> MSEEKVVAVIMVGGPTKGTRFRPLSFNTPKPLIPLAGQPMIHHPISACKKISNLAQIFLIGFYEEREFALYVSSIS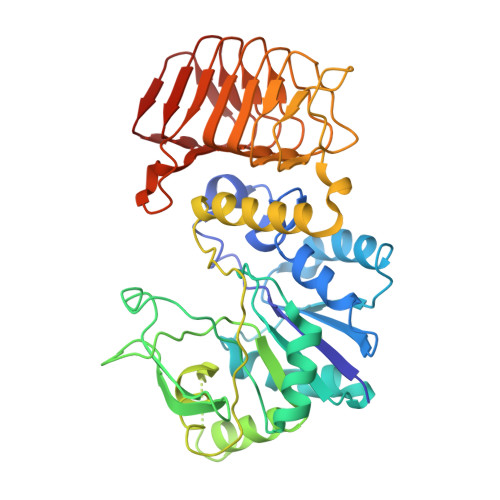NELKIPVRYLKEDKPHGSAGALYYFRDRIMEEKPSHVFLLNCDVCCSFPLQGILDAHRRYGGIGTMLVIKVSAEAASQFGELIADPDTKELLHYTEKPETFVSDLINCGVYVFTSDIFNAIEEVYSQIRDTSSNYQSATRSVPADFVRLDQDILSPLAGKKQLYTYENKDFWEQIKTPGKSLKCSALYLSQFRETSPHILASGDGTNRKPTIIGDVYIHPSVKLHPTAKIGPNVSISANVRVGPGVRLISCIILDDVEIKENAVVINSIIGWKSSIGRWSRVQASGDYNDRLGITILGEAVTVEDEVAVIGSIVLQNKTLNVSVQDDIIL> GDRVADVIESSIGDSVSRALTHALPAPTGQNTQVSSHRLDTGKVPALQAAEIGASSNASDESMIETRCVLNSHSTAETTLDSFFSRAGLVGEIDLPLEGTTNPNGYANWDIDITGYAQMRRKVELFTYMRFDAEFTFVACTPTGEVVPQ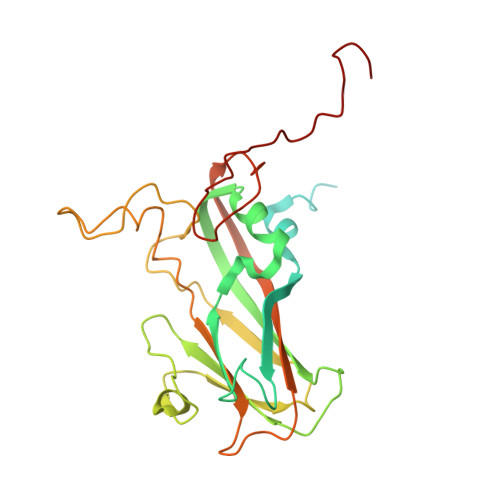LLQYMFVPPGAPKPDSRESLAWQTATNPSVFVKLSDPPAQVSVPFMSPASAYQWFYDGYPTFGEHKQEKDLEYGACPNNMMGTFSVRTVGTSKSKYPLVVRIYMRMKHVRAWIPRPMRNQNYLFKANPNYAGNSIKPTGASRTAITTL>[2x]QILPIRFQEHLQLQNLGINPANIGFSTLTMESDKFICIREKVGEQAQVVIIDMNDPSNPIRRPISADSAIMNPASKVIALKAGKTLQIFNIEMKSKMKAHTMTDDVTFWKWISLNTVALVTDNAVYHWSMEGESQPVKMFDRHSSLAGCQIINYRTDAKQKWLLLT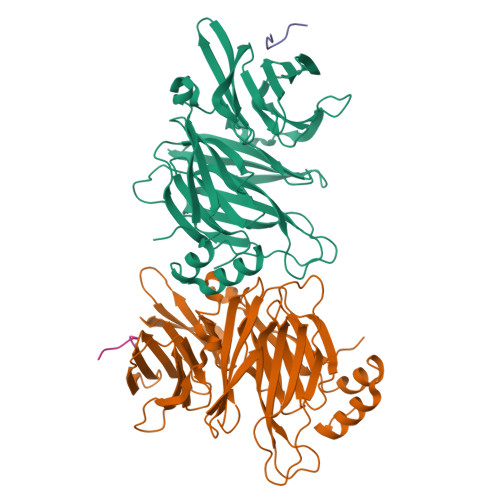GISAQQNRVVGAMQLYSVDRKVSQPIEGHAASFAQFKMEGNAEESTLFCFAVRGQAGGKLHIIEVGTPPTGNQPFPKKAVDVFFPPEAQNDFPVAMQISEKHDVVFLITKYGYIHLYDLETGTCIYMNRISGETIFVTAPHEATAGIIGVNRKGQVLSVCVEEENIIPYITNVLQNPDLALRMAVRNNLAG;>[2x]DTNLIEFE> MPFCGGRPEDGWHHGSIHDMDYPLLGAMAAICSVFIGGSGAWMLYRLDLGLGYSCKPHHSGYAPEANSFSALSCLVSGTIYAAKTFDFFDGGGTPFSFNWYWYLDYVFTCPLILLDVLYTLEIPHKLRFVFAVIITLWCGVAAFVTPSAFRFGYYAVGCVWFVPFSFSLLRHVKQRYQVYPPKCQKLLFWACTIFFGFWPLFPILFLFSWLGTGHIDQQAFTIIHAFLDLFCKTVFGLIMTFFRLELEEHTEVLGLPLNEPKGKH

Kalium channelrhodopsin 1 from Hyphochytrium catenoides (HcKCR1) is a light-gated channel used for optogenetic silencing of mammalian neurons. The genome of H. catenoides also encodes a highly homologous cation channelrhodopsin (HcCCR), a Na+ channel with >100-fold larger Na+ to K+ permeability ratio. Here, we use cryo-electron microscopy to determine atomic structures of these two channels embedded in peptidiscs to elucidate structural foundations of their dramatically different cation selectivity. Together with structure-guided mutagenesis, we show that K+ versus Na+ selectivity is determined at two distinct sites on the putative ion conduction pathway: in a patch of critical residues in the intracellular segment (Leu69/Phe69, Ile73/Ser73 and Asp116) and within a cluster of aromatic residues in the extracellular segment (primarily, Trp102 and Tyr222).

Remarkably, this third channel that we named HcCCR is Na+ selective, with a relative permeability ratio PK/PNa > 100-fold smaller than that of HcKCR14. HcCCR is further characterized by a smaller relative permeability to protons compared to Na+ than that of typical chlorophyte CCRs, and so is potentially useful as an optogenetic tool for neuronal activation that is less likely to produce undesirable acidification of the cytoplasm. On the outer surface of the HcCCR trimer 21 sterol lipids are bound, which all were modeled as cholesterols. In HcKCR1, the Asp116 side chain is H-bonded to two water molecules close to Thr120 and Ile73 in the nearby cavities. In HcCCR, the water molecule is H-bonded to Ser73 instead, and the other water is missing. This is likely caused by the bulky aromatic side chain of Phe69 located in the interface between TM2 and TM3 (Leu69 in HcKCR1), which also influences the position of Asp116. A possible mechanism for this selectivity is that in HcCCR, Ser73 directs its side chain towards the carboxylate group of Asp116. The distance between the OH group of Ser73 and the COOH group of the Asp116 side chain is 6.2 Å. It is possible that in the open state, these two residues stabilize a Na+ ion in between them, whereas this tight coordination may be unfavorable for K+, thereby substitution of Ile73 with a serine diminished K+ selectivity. The S73I mutation increased K+ selectivity of HcCCR5, indicating that the polar side chain protruding into the cavity is a determinant for Na+ selection. Presence of Y222 instead of T222 in HcKCR1 occludes the channel pore compared to HcCCR.>YNGNPFEGVQLWANNYYRSEVHTLAIPQITDPALRAAASAVAEVPSFQWLDRNVTVDTLLVQTLSEIREANQAGANPQYAAQIVVYDLPDRDCAAAASNGEWAIANN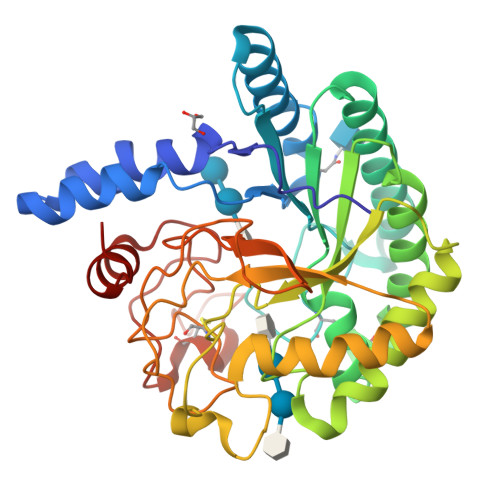GVNNYKAYINRIREILISFSDVRTILVIEPDSLANMVTNMNVPKCSGAASTYRELTIYALKQLDLPHVAMYMDAGHAGWLGWPANIQPAAELFAKIYEDAGKPRAVRGLATNVANYNAWSVSSPPPYTSPNPNYDEKHYIEAFRPLLEARGFPAQFIVDQGRSGKQPTGQKEWGHWCNAIGTGFGMRPTANTGHQYVDAFVWVKPGGECDGTSDTTAARYDYHCGLEDALKPAPEAGQWFNEYFIQLLRNANPPF[2x]> AKNVGILAMDIYFPPTCVQQEALEAHDGASKGKYTIGLGQDCLAFCTELEDVISMSFNAVTSLLEKYKIDPKQIGRLEVGSETVIDKSKSIKTFLMQLFEKCGNTDVEGVDSTNACYGGTAALLNCVNWVESNSWDGRYGLVICTDSAVYAEGPARPTGGAAAIAMLIGPDAPIVFESKLRGSHMAHVYDFYKPNLASEYPVVDGKLSQTCYLMALDSCYKHLCNKFEKLEGKEFSINDADYFVFHSPYNKLVQKSFARLLYNDFLRNASSIDEAAKEKFTPYSSLSLDESYQSRDLEKVSQQLAKTYYDAKVQPTTLVPKQVGNMYTASLYAAFASLVHNKHSDLAGKRVVMFSYGSGSTAT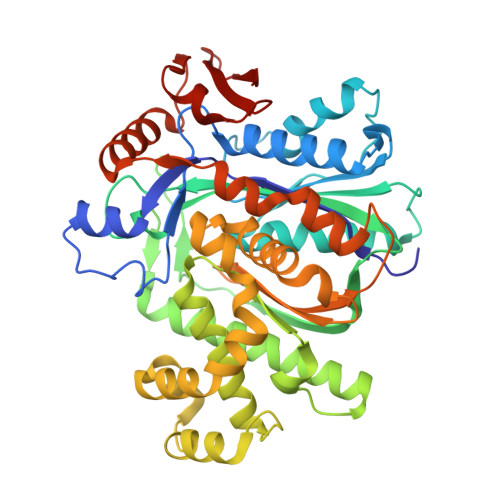MFSLRLCENQSPFSLSNIASVMDVGGKLKARHEYAPEKFVETMKLMEHRYGAKEFVTSKEGILDLLAPGTYYLKEVDSLYRRFYGKK>MEGEVIHRYKVNGFKLFGLPTPKNNTILGVLGKNGVGKTTVLKILAGEIIPNFGDPNSKVGKDEVLKRFRGKEIYNYFKELYSNELKIVHKIQYVEYASKFLKGTVNEILTKIDERGKKDEVKELLNMTNLWNKDANILSGGGLQRLLVAASLLREADVYIFDQPSSYLDVRERMNMAKAIRELLKNKYVIVVDHDLIVLDYLTDLIHIIYGESSVYGRVSKSYAARVGINNFLKGYLPAENMKIRPDEIK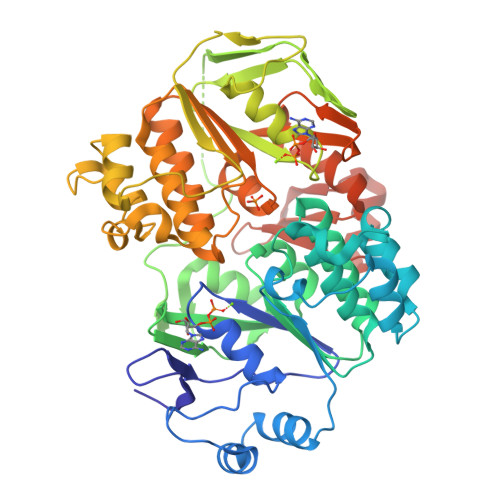FMLKEVSDLDLSKDLKTKMKWTKIIKKLGDFQLVVDNGEAKEGEIIGILGPNGIGKTTFARILVGEITADEGSVTPEKQILSYKPQRIFPNYDGTVQQYLENASKDALSTSSWFFEEVTKRLNLHRLLESNVNDLSGGELQKLYIAATLAKEADLYVLDQPSSYLDVEERYIVAKAIKRVTRERKAVTFIIDHDLSIHDYIADRIIVFKGEPEKAGLATSPVTLKTGMNEFLRELEVTFRRDAETGRPRVNKIGSYLDRVQKERGDYYSMVLSTQGSIEGRHHHHHH[2x]>SPNIVLFSGSSHQDLSQRVADRLGLELGKVVTKKFSNQETSVEIGESVRGEDVYIIQSGCGEINDNLMELLIMINACKIASSSRVTAVIPCFPYARQDKKDKVGESRAPISAKLVANMLSVAGADHIITMDLHASQIQGFFDIPVDNLYAEPAVLQWIRENIAEWKNCIIVSPDAGGAKRVTSIADRLNVEFALIHKERKKANEVDRMVLVGDVKDRVAILVDDMADTCGTICHAADKLLSAGATKVYAILTHGIFSGPAISRINNAAFEAVVVTNTIPQEDKMKHCTKIQVIDISMILAEAIRRTHNGESVSYLFSHVPL[6x]

Phosphoribosyl pyrophosphate synthetase (PRPS) stands as the first and rate-limiting enzyme in the purine biosynthesis pathway. It catalyzes the pyrophosphorylation of D-ribose-5-phosphate (R5P), obtained from the glucose pentose phosphate pathway (PPP), at the 1’ hydroxyl group position, yielding the catalytic product 5-phosphoribosyl-ɑ-1-pyrophosphate (PRPP). PRPP serves as an essential metabolic intermediate for purine biosynthesis via both de novo and salvage pathways, as well as for the synthesis of pyrimidines, amino acids (tryptophan and histidine), and co-factors (NAD+ and NADP+). Conversely, PRPS2 displays ~94% identity with PRPS1 and shares exactly the same biochemical reaction.

To investigate their distinct catalytic mechanisms, we solved the crystal structure of PRPS2 in complex with R5P, ApCpp (an inactive analog of ATP), and Cd2+ ion (an inactive analog of Mg2+) by co-crystallization. However, the Loop2 region in the catalytic pocket of PRPS2 flipped ~90° compared to that of PRPS1 due to the insertion of 3AA. This conformational alteration ultimately reduced the overall size of the PRPS2 catalytic pocket for substrate access (148 Å3 vs 302 Å3 for that of PRPS2 or PRPS1, respectively) and introduced steric clashes with the C-terminal α12’ helix, leading to its structural disorder in the complex (the prime indicates residues or secondary structures from monomers other than monomer A). Surprisingly, PRPS2 exhibited ~15-fold lower kinetic efficiency (kcat/Km) in R5P or ATP compared to PRPS1. Strikingly, in vitro feedback inhibition assays indicated that the enzymatic activity of PRPS1 was inhibited by GDP with an IC50 value of 706 µM, while that of PRPS2 was unaffected by up to 10 mM GDP, suggesting that PRPS2 was insensitive to feedback inhibition. Indeed, PRPS2 binds with GDP with extremely weak affinity (Kd > 200 µM), whereas PRPS1 bound GDP with a Kd value of 10 µM. In contrast, 3AA in PRPS2 sterically blocked GDP binding at the allosteric site, abolishing the feedback inhibition response of PRPS2. The observations also indicated that the four non-conserved residues of PRPS2 (3AA and Q156’) enable its enzymatic function by bypassing the conventional downstream products allosteric feedback inhibition. PRPS2 utilizes four non-conserved key residues to bypass the typical ADP/GDP allosteric feedback inhibition, enabling sustained excess production of newly synthesized ATP.>[3x]MNRVLYPGTFDPITKGHGDLIERA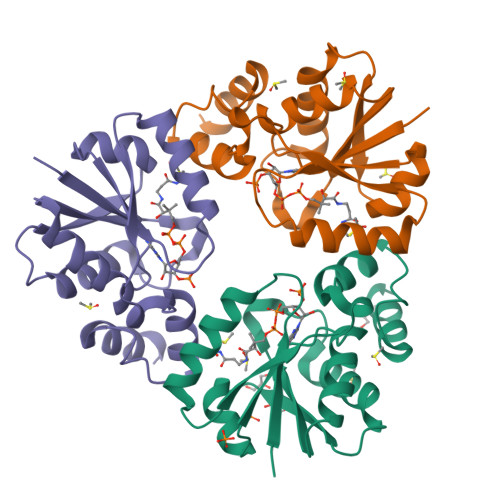SRLFDHVIIAVAASPKKNPLFSLEQRVALAQEVTKHLPNVEVVGFSTLLAHFVKEQKANVFLRGLRAVSDFEYEFQLANMNRQLAPDVESMFLTPSEKYSFISSTLVREIAALGGDISKFVHPAVADALAERFKR>YEANYEDVIKKYKPADAKLDRIAYDWRLHGGVTPVKDQALCGSCWAFSSVGSVESQYAIRKKALFLFSEQELVDCSVKNNGCYGGYITNAFDDMIDLGGLCSQDDYPYVSNLPETCNLKRCNERYTIKSYVSIPDDKFKEALRYLGPISISIAASDDFAFYRGGFYDGECGAAPNHAVILVGYGMKDIYNEDTGRMEKFYYYIIKNSWGSDWG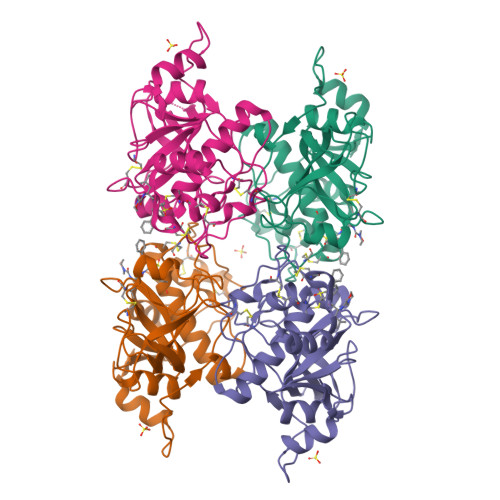EGGYINLETDENGYKKTCSIGTEAYVPLLE[4x]>RLTELREDIDAILEDPALEGAVSGVVVVDTATGEELYSRDGGEQLLPASNMKLFTAAAALEVLGADHSFGTEVAAESAPGRRGEVQDLYLVGRGDPTLSAEDLDAMAAEVAASGVRTVRGDLYADDTWFDSERLVDDWWPEDEPYAYSAQISALTVAHGERFDTGVTEVSVTPAAEGEPADVDLGAAEGYAELDNRAVTGAAGSANTLVIDRPVGTNTIAVTGSLPADAAPVTALRTVDEPAALAGHLFEEALESNGVTVKGDVGLGGVPADWQDAEVLADHTSAELSEILVPFMKFSNNGHAEMLVKSIGQETAGAGTWDAGLVGVEEALSGLGVDTAGLVLNDGSGLSRGNLVTADTVVDLLGQAGSAPWAQTWSASLPVAGESDPFVGGTLANRMRGT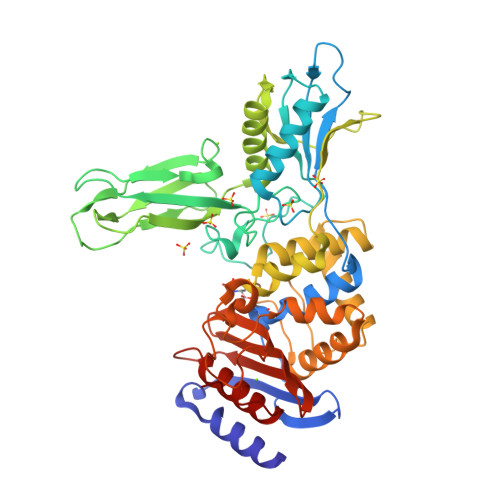AAEGVVEAKTGTMSGVSALSGYVPGPEGELAFSIVNNGHSGPAPLAVQDAIAVRLAEYAGHQAPE[4x]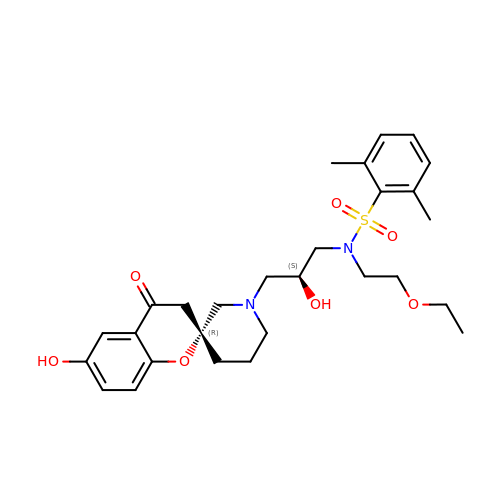N-(2-ethoxyethyl)-N-{(2S)-2-hydroxy-3-[(2R)-6-hydroxy-4-oxo-3,4-dihydro-1'H-spiro[chromene-2,3'-piperidin]-1'-yl]propyl}-2,6-dimethylbenzenesulfonamide | C28 H38 N2 O7 S | ONZIIEDMJXLRAD-NEKDWFFYSA-N>[4x]HMQKVEVFRIPTASPDDISGLATLIDSGKINPAEIVAILGKTEGNGCVNDFTRGFATQSLAMYLAEKLGISREEVVKKVAFIMSGGTEGVMTPHITVFVRKDVAAPAAPGKRLAVGVAFTRDFLPEELGRMEQVNEVARAVKEAMKDAQIDDPRDVHFVQIKCPLLTAERIEDAKRRGKDVVVNDTYKSMAYSRGASALGVALALGEISADKISNEAICHDWNLYSSVASTSAGVELLNDEIIVVGNSTNSASDLVIGHSVMKDAIDADAVRAALKDAGIRSDDEMDRIVNVLAKAEAASSGTVRGRRNTMLDDSDINHTRSARAVVNAVIASVVGDPMVYVSGGAEHQGPDGGGPIAVIARV

The use of cyanuric acid hydrolase to solve this societal problem is being explored and the best candidate for this biotechnological application is the thermostable enzyme from Moorella thermoacetica. Consistent with the “Toblerone fold” observed for these enzymes[8–10], the RMCAH monomer is composed of three concatenated, highly divergent, but structurally homologous domains, which endows the enzyme monomer an internal pseudo-three-fold symmetry (Domains 1, 2). As observed for AtzD and ACAH, the active site of RMCAH lies on the pseudo-three-fold axis within each monomer and is formed by similar sets of residues from all three domains. As observed for ACAH and AtzD, each of the three serine γO atoms is in close proximity to a lysine residue (Lys40, Lys161 and Lys299), generating three pairs of Ser-Lys dyads each from one of the three isostructural domains from the same monomer.

The X-ray crystal structure of the engineered Moorella cyanuric acid hydrolase was determined by molecular replacement and refined to 1.51 Å resolution. All four monomers within the RMCAH tetramer showed clear electron density for a bound ligand in the active site, regardless of whether or not substrate/inhibitor was added during crystallization. The ligand was readily interpreted as malonate, which is a major component of tascimate used in the crystallization condition, and no residual mFo-DFc density was left after further refinement. All four MLA molecules adopt a staggered conformation, in contrast to the planar/eclipsed conformation seen in AtzF. The top-view of MLA shows that the MLA-protein interactions mimic the substrate analogue barbiturate (BAR)-protein interactions at A and B carbonyl-binding sites. The forth oxygen atom is far out of the plane, occupying the position D, (position D) and roughly points to the center of the triangle formed by Ser (83, 231 and 347) γO atoms and is within hydrogen-bonding distance from all three Ser γO atoms. The triangle formed by the three Ser (83, 231 and 347) γO atoms is slightly expanded compared to that in structures with the position D unoccupied. The electron density map clearly reveals one metal ion bound in domain 3 of each monomer in the MLA bound crystals, interacting with the δO of Glu301 carboxyl group, one water molecule, and the carbonyl oxygen atoms of Ala350, Gln353, Pro355, and Gly358. The octahedral coordination is consistent with the presence of Ca2+ in this site.>[2x]MNHKVHMMSQPKPILYYDERSPPVRSCLMLIKLLDIDVELRFVNLFKGEQFQKDFLALNPQHSVPTLVHGDLVLTDSHAILIHLAEKFDEGGSLWP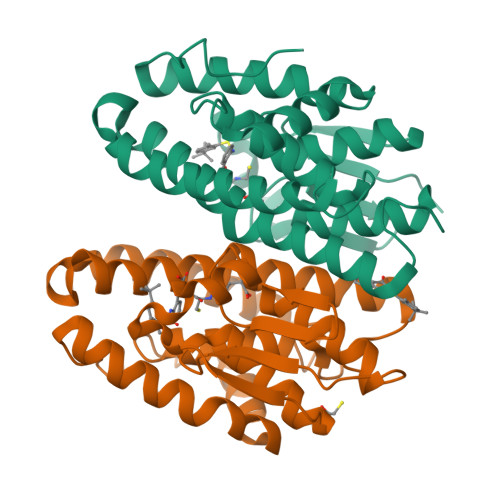QEHAERMKVLNLLLFECSFLFRRDSDFMSAIVRQGFANVDVAHHERKLTEAYIIMERYLENSDFMAGPQLTLADLSIVTTLSTVNLMFPLSQFPRLRRWFTAMQQLDAYEANCSGLEKLRQTMESVGSFQFPSSSAVVTEKVE>MVYVAVLANIAGNFPALTAALEKIEELKEEGYEIEKYYILGNIVGLFPYPREVIEAIKNLAKTSNVKVIRGKYDQLIAMSDPHAGDPKYIDKLEIPDHLKATLKYTWEKLGHEGREYLRDLPIYLVDKIGKNEIFGVYGSPVNPFDGEILPDQPTSYYEAIMRPVKEYEMLLVASPRYPLDAMTMYGRVVCPGSIGFPPAREHKATFALVD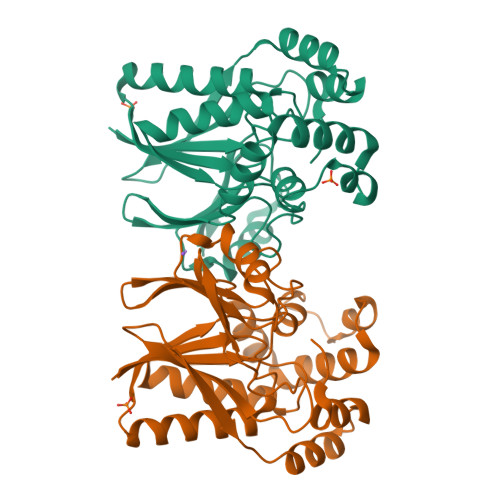AETLKVKFIEVEYDKKIIEDRIKLEKLPEEVIKILYHGGKA[4x]>[2x]SLNNLQNIIYNPVIPFVGTIPDQ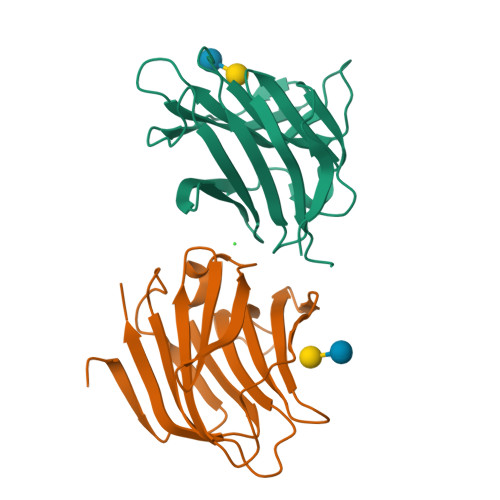LDPGTLIVIRGHVPSDADRFQVDLQNGSSMKPRADVAFHFNPRFKRAGCIVCNTLINEKWGREEITYDTPFKREKSFEIVIMVLKDKFQVAVNGKHTLLYGHRIGPEKIDTLGIYGKVNIHSIGFSFSSDLQ>MTVPTPYEDLLRKIAEEGSHKDDRTGTGTTSLFGQQIRFDLNEGFPLLTTKKVHFHSVVGELLWFLQGDSNVKWLQDNNIRIWNEWADEDGELGPVYGVQWRSWPTPDGRHIDQISGALETLRNNPDSRRNIVSAWNVS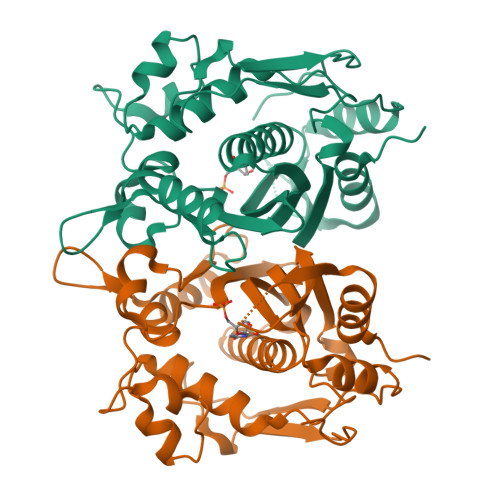ELENMALPPCHLLFQLYVADGKLSCQLYQRSADMFLGVPFNIASYALLTHMFAQQAGLEVGEFIWTGGDCHIYDNHKEQVAEQLSREARPYPTLELNKAASMFEYSFDDITVSGYDPHPLIRGKVAV[4x]>MGSSHHHHHHSSGLVPRGSHMTDLSDVSRTAAAKPPAVPGRGPANKVRFVTAASLFDGHDASINIMRRILQSQGCEVIHLGHNRSVQEVVTAALQEDVQGIAISSYQGGHVEYFKYMIDLLREHGGEHIQVFGGGGGVIVPDEIRELQAYGVARIYSPEDGQRMGLAGMITDMAQRCDIDLTRYAPTTLDTVVAGDRRALAQLITALENGKADPELVSALHAQAKAAAVPVLGITGTGGAGKSSLTDELIRRFRLDQDDALSIAVISIDPSRRKSGGALLGDRIRMNAINHPNIFMRSLATREAGSEISQALPDVIAACKAARFDLVIVETSGIGQGDAAIVPHVDLSLYVMTPEFGAASQLEKIDMLDFADFVAINKFDRKGAQDAWRDVAKQV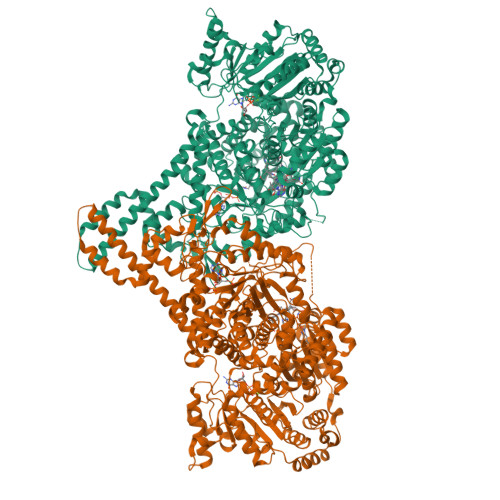QRNREQWHSRAEDMPVYGTQASRFNDDGVTMLYQGLVGALGARGMSLKPGTLPNLEGRISTGQNVIVPPARSRYLAELADTVRAYHRRVVAQSKLARERQQLRAAHDMLQGAGHESAALETLASERDVSLGAVERKLLAMWPQMQQAYSGDEYVVKIRDKEIRTGLISTTLSGTKIRKVVLPRFEDEGEILKWLMRENVPGSFPYTAGVFAFKREGEDPTRMFAGEGDAFRTNRRFKLVSEGMEAKRLSTAFDSVTLYGEDPHERPDIYGKVGNSGVSIATLEDMKVLYDGFDLTNPSTSVSMTINGPAPTILAMFMNTAIDQQIDRFRADNGRDPTADEEAKIRAWVLQNVRGTVQADILKEDQGQNTCIFSTEFSLKVMGDIQEYFVHHQVRNFYSVSISGYHIAEAGANPISQLAFTLANGFTYVEAYLARGMHIDDFAPNLSFFFSNGMDPEYSVLGRVARRIWAVTMRDKYGANDRSQKLKYHIQTSGRSLHAQEIDFNDIRTTLQALIAIYDNCNSLHTNAYDEAITTPTAESVRRALAIQLIINREWGVAKCENPNQGSFLIEELTDLVEEAVLQEFERIAERGGVLGAMETGYQRGKIQEESLYYEQLKHDGTLPIIGVNTFRNPNGDPTPQTLELARSSEDEKQSQLHRLTEFHGAHQADAEAMLARLRQAVIDNRNVFAVLMDAVRVCSLGQITHALFEVGGQYRRNM[2x]> ASSDTTC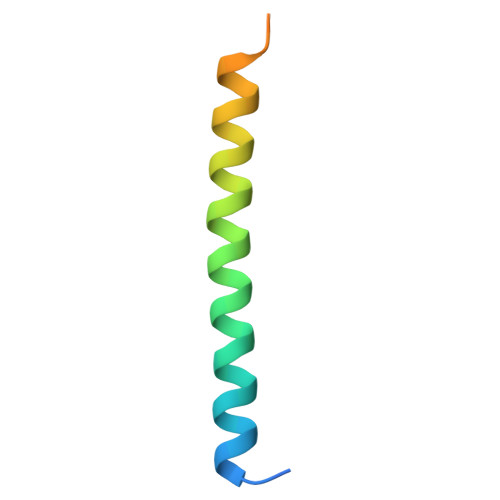ASLTNKLSQHDLADFKKYIKRKFTLMTLLSINNDGFFSNNGGKDEL> ISPIETVPVKLKPGMDGPKVKQWPLTEEKIKALVEICTEMEKEGKISKIGPENPYNTPVFAIKKKDSTKWRKLVDFRELNKRTQDFWEVQLGIPHPAGLKKKKSVTVLDVGDAYFSVPLDEDFRKYTAFTIPSINNETPGIRYQYNVLPQGWKGSPAIFQSSMTKILEPFRKQNPDIVIYQYMDDLCVGSDLEIGQHRTKIEELRQHLLRWGLTTPDKKHQKEPPFLWMGYELHPDKWTVQPIVLPEKDSWTVNDIQKLVGKLNWASQIYPGIKVRQLCKLLRGTKALTEVIPLTEEAELELAENREILKEPVHGVYYDPSKDLIAEIQKQGQGQWTYQIYQEPFKNLKTGKYARMRGAHTNDVKQLTEAVQKITTESIVIWGKTPKFKLPIQKETWETWWTEYWQATWIPEWEFVNTPPLVKLWYQLEKEPIVGAETFYVDGAANRETKLGKAGYVTNRGRQKVVTLTDTTNQKTELQAIYLALQDSGLEVNIVTDSQYALGIIQAQPDQSESELVNQIIEQLIKKEKVYLAWVPAHKGIG;> ETVPVKLKPGMDGPKVKQWPLTEEKIKALVEICTEMEKEGKISKIGPENPYNTPVFAIKKKDSTKWRKLVDFRELNKRTQDFWEVQLGIPHPAGLKKKKSVTVLDVGDAYFSVPLDEDFRKYTAFTIPSINNETPGIRYQYNVLPQGWKGSPAIFQSSMTKILEPFRKQNPDIVIYQYMDDLCVGSDLEIGQHRTKI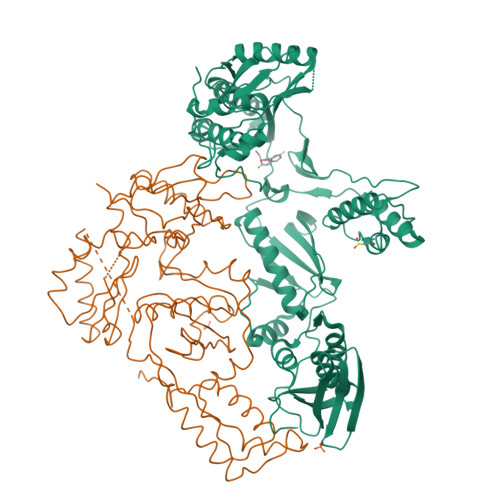EELRQHLLRWGLTTPDKKHQKEPPFLWMGYELHPDKWTVQPIVLPEKDSWTVNDIQKLVGKLNWASQIYPGIKVRQLCKLLRGTKALTEVIPLTEEAELELAENREILKEPVHGVYYDPSKDLIAEIQKQGQGQWTYQIYQEPFKNLKTGKYARMRGAHTNDVKQLTEAVQKITTESIVIWGKTPKFKLPIQKETWETWWTEYWQATWIPEWEFVNTPPLVKLWYQLEKEPIVGAETF> MQQGQMAYDRAITVFSPDGRLFQVEYAREAVKKGSTALGMKFANGVLLISDKKVRSRLIEQNSIEKIQLIDDYVAAVTSGYVADARVLVDFARISAQQEKVTYGSLVNIENLVKRVADQMQQYTQYGGVRPYGVSLIFAGIDQIGPRLFDCDPAGTINEYKATAIGSGKDAVVSFLEREYKENLPEKEAVTLGIKALKSSLEEGEELKAPEIASITVGNKYRIYDQEEVKKF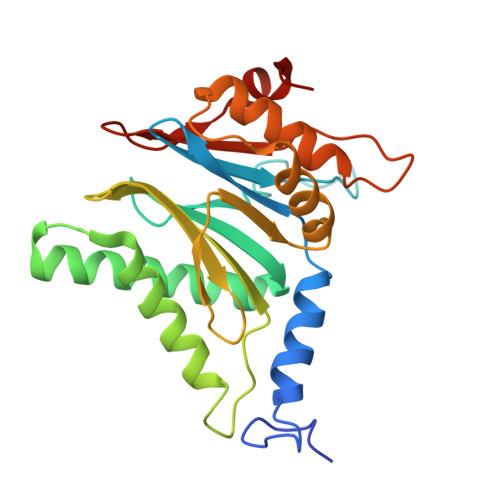L[(2~{R},4~{S})-4-(3-chlorophenyl)pyrrolidin-2-yl]-(4-thieno[2,3-c]pyridin-7-ylpiperazin-1-yl)methanone 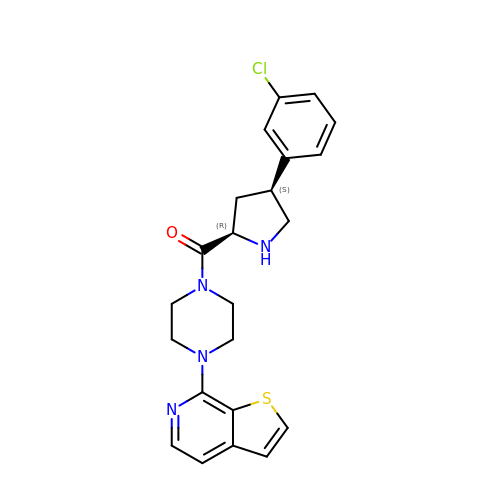| C22 H23 Cl N4 O S | YMNUWCFQVRYQGA-IEBWSBKVSA-N> MEAYLNKIDKIEPSDQKIKEEYNKFKYDITKQAIESLRERIPKRIIFFNNLVNVNSEPGSILNVNDLDGVSYKYKINKIEENVRKKHKGNNSSDFDEREKKK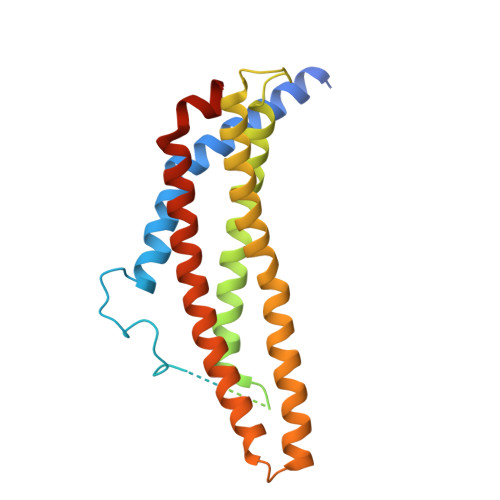DSLDGHVKHFSNNEDSKLIIDDKVLYTHYVPSHKQIYLELEKIKTYASELIEIIGNIKLWIQLNVPRIEDGNNFGVGIQEEAIQELARVEESAFNLYDAIVKYYMERAKISTKVLKYPNVSDYQEAVRELDEKEWIHIKITIVDMRNNYIMLYDLLYKNWEKVVKPKNEDAHHRMTF>MASWSHPQFEKGADDDDKVPDPTSVDSVKYSKIKGIPKLDDANDAGGKHSLECTLILTEGDSAKSLAVSGLGVIGRDRYGVFPLRGKILNVREASHKQIMENAEINNIIKIVGLQYKKSYDDAESLKTLRYGKIMIMTDQDQDGSHIKGLLINFIHHNWPSLLKHGFLEEFITPIVKASKNKQELSFYSIPEFDEWKKHIENQKAWKIKYYKGLGTSTAKEAKEYFADMERHRILFRYAGPEDDAAITLAFSKKKIDDRKEWLTNFMEDRRQRRLHGLPEQFLYGTATKHLTYNDFINKELILFSNSDNERSIPSLVDGFKPGQRKVLFTCFKRNDKREVKVAQLAGSVAEMSAYHHGEQALMMTIVNLAQNFVGSNNINLLQPIGQFGTRLHGGKDAASPRYIFTMLSTLARLLFPAVDDNLLKFLYDDNQRVEPEWYIPIIPMVLINGAEGIGTGWACKLPNYDAREIVNNVRRMLDGLDPHPMLPNYKNFKGTIQELGQNQYAVSGEIFVVDRNTVEITELPVRTWTQVYKEQVLEPMLNGTDKTPALISDYKEYHTDTTVKFVVKMTEEKLAQAEAAGLHKVFKLQTTLTCNSMVLFDHMGCLKKYETVQDILKEFFDLRLSYYGLRKEWLVGMLGAESTKLNNQARFILEKIQGKITIENRSKKDLIQMLVQRGYESDPVKAWKEAQEKAAEEDETQNQHDDSSSDSGTPSGPDFNYILNMSLWSLTKEKVEELIKQRDAKGREVNDLKRKSPSDLWKEDLAAFVEELDKVESQEREDGAPGFSSISAHHHHHHHHHH[2x]

Top2s in mammalian cells can be divided into two subtypes which are type IIα (Top2α) and IIβ (Top2β). And Top2β is associated with DNA repair and transcription. Especially, site-specific cleavage of DNA by human topoisomerases IIβ (hTop2β) has been reported to be necessary to activate the transcription of some genes. Beyond the vital cellular functions, Top2s are considered as an important target protein for some of the most active drugs for the treatment of human cancers.

Using the well-established system for hTop2β crystal growth, the crystal of hTop2β cleavage complex containing two monomers of hTop2β and cleaved DNA chain was obtained under the action of compound C-Bi with the resolution of 2.54 Å. All DNA base pairs were visible in the electron density maps. However, no molecule of compound C-Bi was observed in the stabilized hTop2β cleavage complex structures. The structure of the hTop2β-DNA binary complex revealed a looser assembly pattern than in hTop2β-DNA-etoposide ternary complex and other DNA-bound structures. However, the changes of structure were mainly located in the DNA-gate, and there was no obvious change in the C-gate. The distance between drug-binding sites Arg503 of the two monomers was 26.62 Å in hTop2β-DNA-etoposide ternary complex and 34.54 Å in hTop2β-DNA binary complex, respectively. In this work, perhaps because of the loose assembly of monomers, the distance between Arg503 and +5 guanine base was increased, and no hydrogen bond was observed. Similarly, the phosphotyrosyl linkage that should existed between +1 nucleotide and active site residue Tyr821’ was weaken. DNA-intercalating isoleucine (Ile872) still bound between the +8 and +9 bases. DNA chains were more significantly twisted, and some bases could not be paired with each other (+1/+4). Lack of base-pairing and torsion of the DNA chains leads to an inability to re-ligate the DNA break, thus preventing repair of the DNA damage.>MQNERSEQSMPGMPAPGLPAGFERRFSRRYAQLDDVRLHYVTGGPDDGEMVVLLHGWPQTWYTWRHVMPALAEDGYRVVAVDYRGAGESDKPLGGYDKASMAGDIRALVHQLGATRIHLVGRSIGVMVAYAYAAQWPTEIVKLAMLDVPVPGTRIWDEAKASADPQIWHFGLHQQRDIAEMLIAGKERAYILDFYKKRTHVALSNDDIAVYADAYAAPGALRAGFELYRAFPQDETRFKAFMKHKLPMPVLALAGDKSNGAKELDMARELALDVRGAVAPNTGHWLPDENPAFLTRQLLDFFREAASGR[8x]

Here we report the biochemical and structural characteristics of Cfl1 and Cfl2, two Cif-like epoxide hydrolases from Burkholderia cenocepacia. EHs that belong to the α/β hydrolase superfamily of enzymes utilize an Asp-His-Asp/Glu catalytic triad to open the epoxide ring substrate and release the vicinal diol product. Cfl1 and Cfl2 also appear to utilize a Cif-like His-Tyr epoxide ring-opening pair instead of the classical Tyr-Tyr pair. While Cif and aCif exist as constitutive dimers, our hydrodynamic and structural studies revealed that Cfl1 and Cfl2 exist as octamers and decamers, respectively, by forming rings of dimers.

Cfl1 amino-acid sequence alignment with Cif suggests that Asp123 is responsible for the nucleophilic attack that opens the epoxide ring. To test this hypothesis, we expressed and purified a mutant Cfl1 in which Asp123 was substituted with a serine (Cfl1-D123S). Although hydrolysis of R–SO by the mutant formally crosses the threshold of statistical significance, the low absolute level of hydrolysis measured is unlikely to be catalytically meaningful and is sharply decreased compared to the wild-type hydrolysis of R–SO, consistent with our mechanistic hypothesis. The four epoxides vary in length, number of double bonds, and the position of the epoxide moiety along the hydrocarbon chain. Wild-type Cfl1 showed significantly more activity against these epoxides compared to Cfl1-D123S. To that end, we determined the crystal structure of Cfl1-D123S. Data were obtained to 2.15 ​Å resolution, although the UCLA Diffraction Anisotropy Server reports modest anisotropy (2.2, 2.5, and 2.3 ​Å along a∗, b∗, and c∗, respectively) (Strong et al., 2006). As a result, we refined translation, libration, and screw (TLS) rotation parameters, which created a significant improvement in the Rfree value without overfitting, as judged by Rfree-Rwork. The RMSD of main-chain atoms between wild-type Cfl1 and Cfl1-D123S monomers is 0.2 ​Å. Closer inspection of the mutant enzyme's active site shows that, apart from the D123S substitution, the active site is largely unchanged compared to the wild-type enzyme (inset).> GPLGSPEFEDDLYRQSLEIISRYLREQATGSKDSKPLGEAGAAGRRALETLRRVGDGVQRNHETAFQGMLRKLD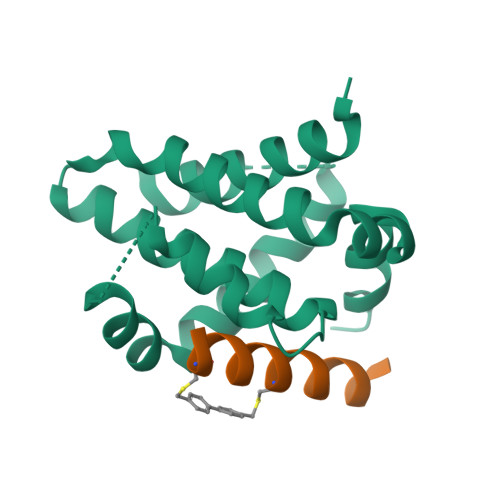IKNEGDVKSFSRVMVHVFKDGVTNWGRIVTLISFGAFVAKHLKSVNQESFIEPLAETITDVLVRTKRDWLVKQRGWDGFVEFFHVQDLEGG;> XAACLRRIGDCVNLRQKLLNX(2S,3R,4E)-2-(dodecanoylamino)-3-hydroxyoctadec-4-en-1-yl dihydrogen 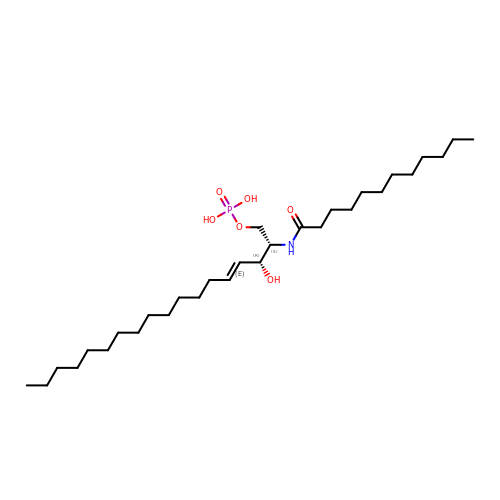phosphate | C30 H60 N O6 P | KXEMZGPJXBKYJP-VARSQMIESA-N(2S)-2-[(3R)-3-(acetylamino)-3-(2-methylpropyl)-2-oxopyrrolidin-1-yl]-N-{(1R,2S)-3-(3,5-difluorophenyl)-1-hydroxy-1-[(3R)-1,2,3,4-tetrahydroisoquinolin-3-yl]propan-2-yl}-4-phenylbutanamide 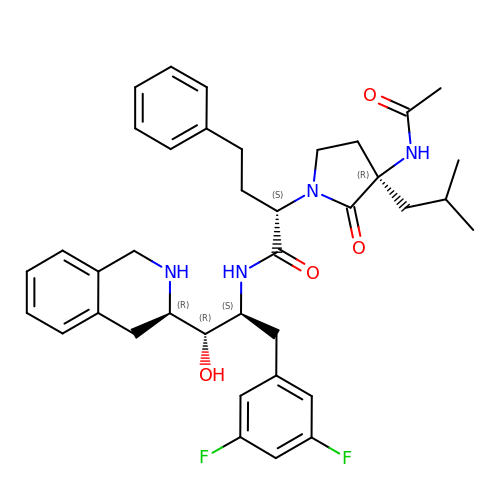| C38 H46 F2 N4 O4 | JJJDOYFRIVNWHV-WUCUQKTKSA-N Dihydroxypropanesulfonate (DHPS), a globally abundant organosulfur compound, serves as an ecologically important currency for nutrient and energy transfer from phytoplankton to bacteria in the ocean. A novel chiral-selective DHPS catabolic pathway was identified in marine Roseobacteraceae strains, where HpsO and HpsP dehydrogenases at the gateway to DHPS catabolism act specifically on R-DHPS and S-DHPS, respectively. R-DHPS is also a substrate for the dehydrogenase HpsN. All three dehydrogenases generate stable hydrogen bonds between the chirality-center hydroxyls of DHPS and highly conserved residues, and HpsP also form coordinate–covalent bonds between the chirality-center hydroxyls and Zn2+, which determines the mechanistic basis of strict stereoselectivity.

The RpHpsN structure consists of four molecules arranged as a tetramer in an asymmetric unit. Each RpHpsN monomer contains two smaller domains (domains: C and D) and two large domains (domains: A and B) harboring Rossmann-like folds. Sequence-based functional prediction suggested that RpHpsN belongs to the aldehyde dehydrogenase (ALDH) superfamily and is a metalloenzyme containing a Zn2+-binding region. Although the electron density indicative of Zn2+ was not observed in protein structure of RpHpsN, ICP-MS analysis confirmed the presence of Zn2+ and Mn2+ in the protein. RpHpsN recovered 60% and 88% of native enzymatic activities after addition of Zn2+ and Mn2+ to metal-chelated reaction mixtures, respectively, demonstrating that RpHpsN is a metal-dependent enzyme. The reaction product of RpHpsN catalyzing R-DHPS was identified as sulfolactate by its retention time, exact mass of the [M-H]− ion, and MS/MS fragmentation pattern. The C3-OH of R-DHPS could form hydrogen bond interactions with NE2 of His320 and O of His360, respectively. Residue His320 from RpHpsN is conserved in l-histidinol dehydrogenase (His327) from E. coli MC1061, where it functions as a general base participating in catalysis, implying a potentially similar function for His320 in RpHpsN. Mutagenesis His320Ala of RpHpsN was conducted and completely abolished enzymatic activity toward R-DHPS, indicating the essential catalytical function of His320 for R-DHPS catalyzation. The chirality-center C2-OH of R-DHPS, oriented toward reverse direction of NAD+ and formed a hydrogen bond with OD2 of Asp353.

>[4x]MTIEYLKKASLTSKSDASDVQETVRAILADIEAGGDQVALDYAAKFDRYEGSIILSPEEIEAACAKVPEKLKADIRFAHDNVRRFAETQKATLTDVELEVVPGVITGQKAIPVDAAGCYVPGGRYSHIASAIMTVTTAKVAGCKHIMACSPPRPGVGVAPAIVYAAHICGADTIMAIGGVQGVASMAFGLFGLPKAKILVGPGNQFVAEAKRMLFGRVGIDMIAGPTDSLILADRTADPHIVTTDLVSQAEHGYNSPVWLVTDDRALAEKVIEMIPSYIADLPEVNRDNAAAAWRDYAEVILCADREEMAATSDRYAPEHLTVMAEDLDWWLDRLSCYGSLFLGEESTVSYGDKAAGTNHVLPTSGAASYTGGLSVHKYMKIVTWQRGTREGYKPVAEATARIARLE Here, we elucidated the crystal structure of SAYabJ from Staphylococcus aureus Mu50 and its function as a ribonuclease after chlorination. SAYabJ is classified as a member of the typical RidA subfamily by sequence analysis, and all six footprint residues (Tyr16, Ser29, Asn87, Arg101, Cys103, and Glu116) are conserved. The crystal structure reveals that SAYabJ exists as a compact homotrimer, which is consistent with the results of size-exclusion chromatography. We first identified SAYabJ as a ribonuclease that is activated after chlorination.

The 1.75-Å crystal structure of SAYabJ has clear electron density for 125 amino acids. Each SAYabJ monomer consists of a β-sheet and two α-helices. Six β-strands, β1 (residues 2–4), β2 (residues 19–22), β3 (residues 25–28), β4 (residues 70–77), β5 (residues 100–105), and β6 (residues 115–122) are aligned in a single sheet, and two α-helices, α1 (residues 45–63) and α3 (residues 80–92) are packed against the β-sheet. The ball-like trimeric structure forms a hole in the center area with a diameter of approximately 10 Å, with ∼20 water molecules positioned in the interior. The β-strands (β2–β6) form a central barrel with a hollow center that does not completely permeate the protein, and all α-helices are located around the perimeter, solvent exposed. The surface electrostatic potential map shows that positively charged residues predominate at the entry of the center cavity, and negatively charged residues are dominant on the opposite side. Each monomer has a deep pocket on its surface. In the crystal structure of SAYabJ, all six footprint residues are positioned toward the deep pocket on the surface, where they are known to be involved in ligand binding. The surface electrostatic potential distribution of the groove shows a positively charged surface patch comprising Lys78, Lys111, and Arg108. From the mutants study, we have shown that Tyr16, His18, Lys39, Arg101, Cys103, and Lys111, which are predicted as the potential nucleic acid binding groove, are important for the chlorinated SAYabJ performing ribonuclease activity.

>GAASMKIINTTRLPEALGPYSHATVVNGMVYTSGQIPLNVDGKIVSADVQAQTKQVLENLKVVLEEAGSDLNSVAKATIFIKDMNDFQKINEVYGQYFNEHKPARSCVEVARLPKDVKVEIELVSKIKEL[6x]>[2x]GSQS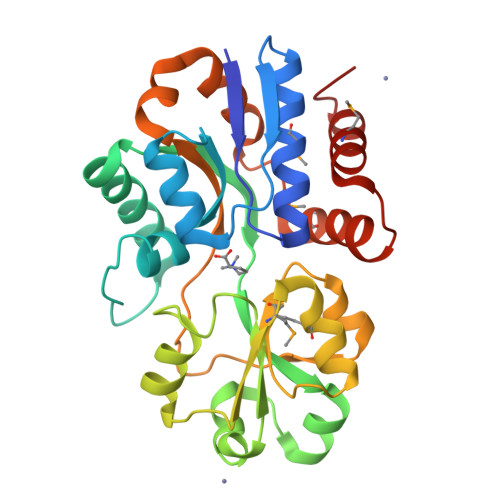SERVVIGSKPFNEQYILANMIAILLEENGYKAEVKEGLGGTLVNYEALKRNDIQLYVEYTGTAYNVILRKQPPELWDQQYIFDEVKKGLLEADGVVVAAKLGFRDDYALAVRADWAEENGVEKISDLAEFADQLVFGSDPEFASRPDGLPQIKKVYGFEFKEVKQMEPTLMYEAIKNKQVDVIPAYTTDSRVDLFNLKILEDDKGALPPYDAIIIVNGNTAKDEKLISVLKLLEDRIDTDTMRALNYQYDVEKKDAREIAMSFLKEQGLVK> VANSVLFPCKYASSGCEITLPHTEKADHEELCEFRPYSCPCPGASCKWQGSLDAVMPHLMHQHKSITTLQGEDIVFLATDINLPGAVDWVMMQSCFGFHFMLVLEKQEKYDGHQQFFAIVQLIGTRKQAENFAYRLELNGHRRRLTWEATPRSIHEGIATAIMNSDC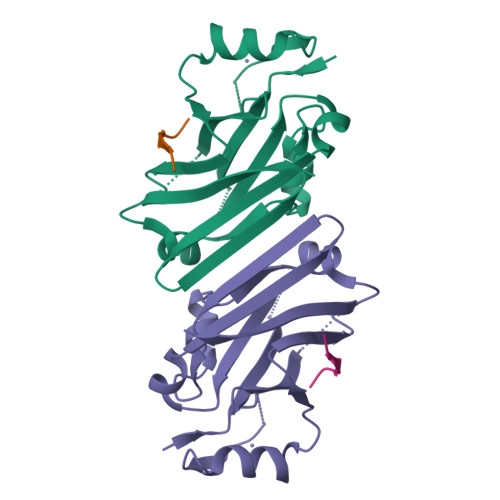LVFDTSIAQLFAENGNLGINVTISMC;> EKPAAVVAPITTG>[14x]MEQAMRERSELARKGIARAKSVVALAYAGGVLFVAENPSRSLQKISELYDRVGFAAAGKFNEFDNLRRGGIQFADTRGYAYDRRDVTGRQLANVYAQTLGTIFT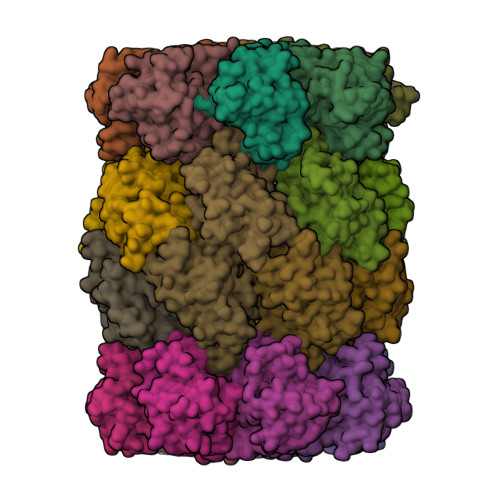EQAKPYEVELCVAEVAHYGETKRPELYRITYDGSIADEPHFVVMGGTTEPIANALKESYAENASLTDALRIAVAALRAGSADTSGGDQPTLGVASLEVAVLDANRPRRAFRRITGSALQALLVDQESPQSDGESSG;>[14x]TTIVALKYPGGVVMAGDRRSTQGNMISGRDVRKVYITDDYTATGIAGTAAVAVEFARLYAVELEHYEKLEGVPLTFAGKINRLAIMVRGNLAAAMQGLLALPLLAGYDIHASDPQSAGRIVSFDAAGGWNIEEEGYQAVGSGSLFAKSSMKKLYSQVTDGDSGLRVAVEALYDAADDDSATGGPDLVRGIFPTAVIIDADGAVDVPESRIAELARAIIESRSGADTFGSDGGEK> MLLQK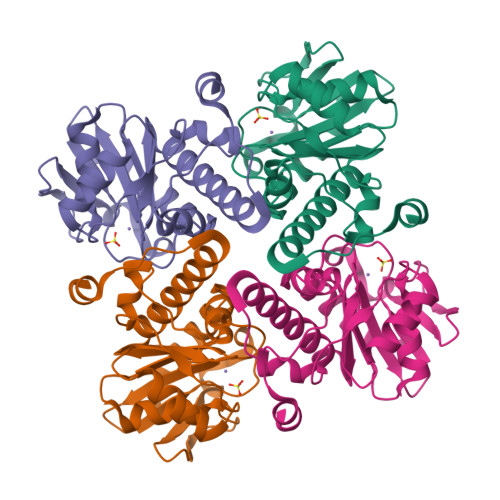EREEIVAYGKKMISSGLTKGTGGNISIFNREQGLVAISPSGLEYYETKPEDVVILNLDGEVIEGERKPSSELDMHLIYYRKREDINALVHTHSPYAKTIASLGWELPAVSYLIAFAGPNVRCAPYETFGTKQLADAAFEGMIDRRAVLLANHGLIAGANNIKMAFTVAEEIEFCAQIYYQTKSIGEPKLLPEDEMENLAKKFEGYGQQYLEHHHHHH> GSMSSERVLSYAPAFKSFLDTSFFQELSRLKLDVLKLDSTCQPLTVNLDLHNIPKSADQVPLFLTNRSFEKHNNKRTNEVPLQGSIFNFNVLDEFKNLDKQLFLHQRALECWEDGIKDINKCVSFVIISFADLKKYRFYYWLGVPCFQRPSSTVLHVRPEPSLKGLFSKCQKWFDVNYSKWVCILDADDEIVNYDKCIIRKTKVLAIRDTSTMENVPSALTKNFLSVLQYDVPDLIDFKLLIIRQNEGSFALNATFASIDPQSSSSNPDMKVSGWERNVQGKLAPRVVDLSSLLDPLKIADQSVDLNLKLMKWRILPDLNLDIIKNTKVLLLGAGTLGCYVSRALIAWGVRKITFVDNGTVSYSNPVRQALYNFEDCGKPKAELAAASLKRIFPLMDATGVKLSIPMIGHKLVNEEAQHKDFDRLRALIKEHDIIFLLVDSRESRWLPSLLSNIENKTVINAALGFDSYLVMRHGNRDEQSSKQLGCYFCHDVVAPTDSLTDRT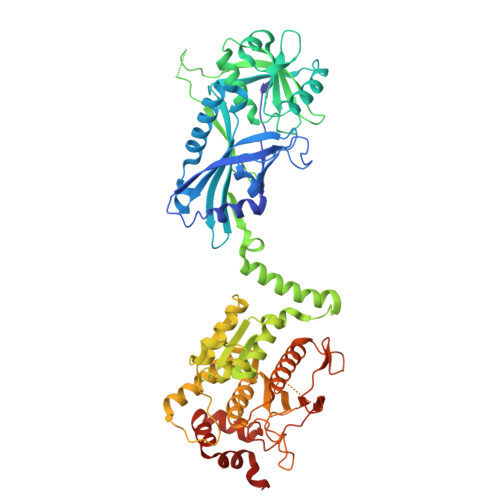LDQMCTVTRPGVAMMASSLAVELMTSLLQTKYSGSETTVLGDIPHQIRGFLHNFSILKLETPAYEHCPACSPKVIEAFTDLGWEFVKKALEHPLYLEEISGLSVIKQEVER> GMGFTIDIKSFLKPGEKTYTQRCRLFV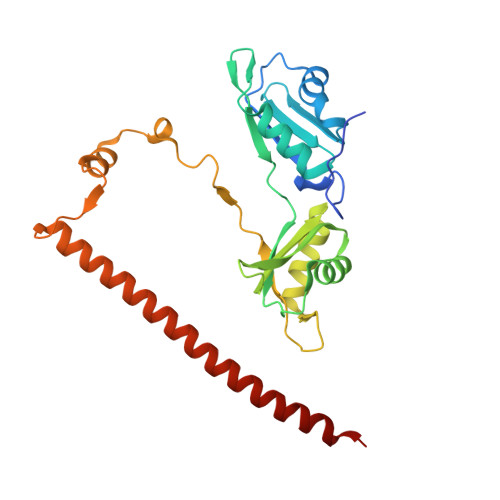GNLPTDITEEDFKRLFERYGEPSEVFINRDRGFGFIRLESRTLAEIAKAELDGTILKSRPLRIRFATHGAALTVKNLSPVVSNELLEQAFSQFGPVEKAVVVVDDRGRATGKGFVEFAAKPPARKALERCGDGAFLLTTTPRPVIVEPMEQFDDEDGLPEKLMQKTQQYHKEREQPPRFAQPGTFEFEYASRWKALDEMEKQQREQVDRNIREAKEKLEAEMEAARHEHQLMLM3-[[(1R,2R,4aS,8aR)-2-methyl-1,2,4a,5,6,7,8,8a-octahydronaphthalen-1-yl]carbonyl]-5-(4-hydroxyphenyl)-4-oxidanyl-1H-pyridin-2-one | C23 H25 N O4 | 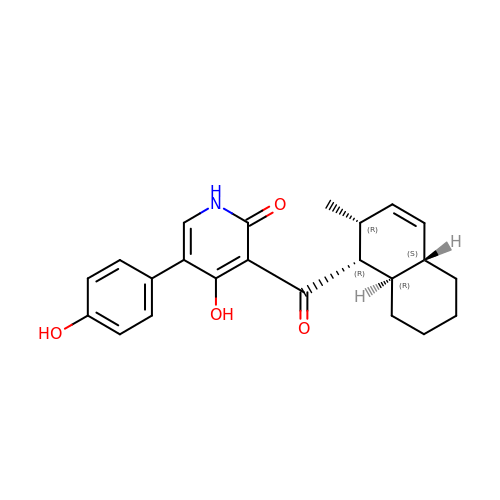GLNYCQCUCACIJN-QOIYZWAUSA-N Type II AFP is a 14 kDa globular protein composed of both α-helices and β-strands with five disulfide-bonds. The Ca2+-dependent type II AFPs have been identified from Japanese smelt (Hypomesus nipponensis) (jsAFP), rainbow smelt (Osmerus mordax) (smeltAFP), and Atlantic herring (Clupea harengus) (hAFP). In the present study, we determined the crystal structure of a Ca2+-dependent type II AFP from Japanese smelt denoted jsAFP, and made a structural comparison between its Ca2+-bound and -free forms to elucidate its ice-binding mechanism via Ca2+ ion. The obtained data revealed that binding of Ca2+ does not affect overall structural motif of jsAFP but alters its side-chain conformation as well as its rigidity of the Ca2+-binding loop, facilitating a formation of the polypentagonal ice-like waters on the IBS.

The X-ray structure of jsAFP in the Ca2+-bound state was determined with preparation of its crystal in a solution composed of 0.1 M sodium acetate buffer (pH 7.0), 0.2–0.25 M ammonium sulfate, 8% PEG 3350, and 2 mM CaCl2. The overall structure of the Ca2+-bound jsAFP is composed of two alpha-helices (α1 and α2), eight beta-strands (β1–β8) and four loop regions (L1: C69–W75, L2: W77–T81, L3: C89–Q92, L4: D94–E99). The molecule is further stabilized by five disulfide-bonds (C4–C15, C32–C125, C69–C100, C89–C111 and C101–C117) and a hydrophobic core composed of aromatic and aliphatic residues. A Ca2+ ion was located at the molecular surface between β7 and a loop segment L3–L4 of jsAFP, and was coordinated with the side-chain oxygen atoms of Q92, D94 E99, D113, D114, a backbone oxygen atom of D114, and an oxygen atom of a water molecule. Significantly, a total of 16 waters are organized into an ice-like arrangement on the putative IBS (left). They construct at least five pentagonal rings (PI~PV) and one hexagonal ring (HI) that are next to each other, in which a few oxygen atoms of the side-chain groups of jsAFP are also involved. The side-chain OH-groups of T96 and T98 are therefore thought to play a crucial role to anchor the water molecules via hydrogen-bonds, and function as a scaffold for the polypentagonal formation. The obtained docked model showed that waters 1, 3, 4, 5, 6, 10 (cyan) as well as the side-chain oxygen atoms of D94 and E99 perfectly match to the waters constructing the 1st prism plane, whose RMSD was less than 1.0 Å. The B-factors along the sequence of the Ca2+-bound jsAFP (cyan line) is lower than that of the Ca2+-free form (orange line), suggesting that 1 mol of Ca2+-binding rigidifies the overall structure of jsAFP. Indeed, the IBS of most the AFPs tends to be hydrophobic. It is speculated that the Ca2+ ion in the jsAFP structure plays a role to neutralize the electric charge of the acidic residues of the IBS, which increases its hydrophobicity to lead and organize the polypentagonal ice-like waters.

> HHHHHHADECPTDWKLFDGTCYLFNPSVLHWADAQESCMKEGASLASIHSLEQYTFVKELTTAALTPSWLGGGDCQVSTRWFWMDGTSMDFTDWCYAQPDTTLTECCIQMNVGVGKCWDDTPCTHLHSSICAKTST>[2x]FTCPECRPELCGDPGYCEYGTTKDACDCCPVCF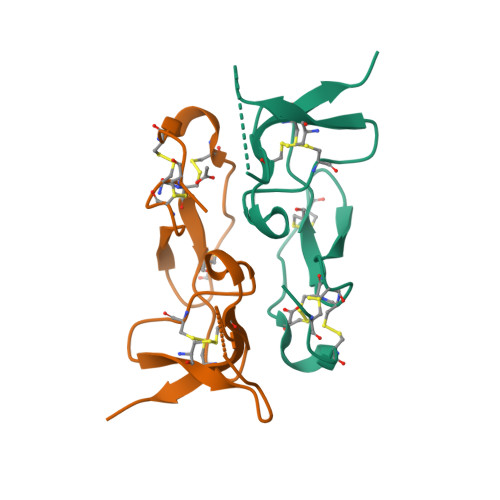QGPGGYCGGPEDVFGICADGFACVPLVGERDSQDPIVGTCVKIP Following an extensive screen of prokaryotic homologues with high (>40%) amino acid sequence identity to eukaryotic SLC7 transport proteins, we identified a suitable candidate from the thermophilic bacterium Geobacillus Kaustophilus, GkApcT. To address these questions, we determined the crystal structure of a close prokaryotic SLC7 homologue in complex with bound l-alanine and l-arginine ligands and studied its transport mechanism using in vitro biochemical assays. GkApcT was determined to be proton-coupled, with uptake of l-[3H]-Ala observed in the presence of a membrane potential, negative inside and a pH gradient, alkaline inside. Crystal structures of APC superfamily transporters have revealed a conserved ‘5 + 5 inverted topology’ fold, wherein the first five TM helices are related to the second five helices via a pseudo two-fold symmetry axis running parallel to the plane of the membrane.

Crystals were eventually obtained in the presence of l-Alanine and cholesterol doped monoolein, and diffracted X-ray to 2.86 Å. GkApcT adopts a ligand bound inward occluded state with solvent filled cavities extending towards the bound ligand from either side of the membrane. Clear electron density was observed in the structure for the bound ligand, l-Ala. A conserved aromatic side chain on TM6, Phe231 and threonine, Thr43, on TM1 provide the main steric occlusion that seals the binding site from the extracellular side of the membrane. In contrast, intracellular access is less obstructed, with only a thin occlusion separating the ligand binding site from the solvent filled cytoplasmic tunnel leading to the inside of the cell. This thin gate is constructed principally from hydrophobic side chains on TM8, Met321, and TM6A, Ile234 and Glu115 on TM3. The amino group predominantly interacts with the carbonyl groups of Phe231, Ala232 and Ile234 from TM6 with one interaction to Ile40 from TM1. In contrast, the carboxyl group interacts with TM1, making polar contacts to the amino groups of Thr43 and Gly44. In contrast, in GkApcT we observe the α-carboxylate group of l-Ala interacting with a well-ordered water molecule, in addition to the backbone amide groups of Thr43 and Gly44. The maps were of sufficient quality to allow us to identify this helix as YneM, which has recently been renamed as MgtS, a single spanning transmembrane protein from Escherichia coli. In our structure, we observed density for a cholesterol molecule in this pocket.

> MNLFRKKPIQLLMKESGAKGASLRKELGAFDLTMLGIGAIIGTGIFVLTGVAAAEHAGPALVLSFILSGLACVFAALCYAEFASTVPVSGSAYTYSYATFGELIAWILGWDLILEYGVASSAVAVGWSGYFQGLLSGFGIELPKALTSAYDPAKGTFIDLPAIIIVLFITFLLNLGAKKSARFNAVIVAIKVAVVLLFLAVGVWYVKPENWTPFMPYGFSGVATGAATVFFAYIGFDAVSTAAEEVRNPQRDMPIGIIVSLLVCTLLYIAVSLVLTGIVPYEQLNVKNPVAFALNYIHQDWVAGFISLGAIAGITTVLLVMMYGQTRLFYAISRDGLLPKVFARISPTRQVPYVNTWLTGAAVAVFAGIIPLNKLAELTNIGTLFAFITVSIGVLVLRKTQPDLKRAFRVPFVPVVPILAVLFCGYLVLQLPAMTWIGFVSWLLIGLVIYFIYGRKHSELNEMARTEEKAG;> MLGNMNVFMAVLGIILFSGFLAAYFSHKWDD>MLESKLKAPVFTARTQGRHYGEFVLEPLERGFGVTLGNPLRRILLSSIPGTAVTSVYIEDVLHEFSTIPGVKEDVVEIILNLKELVVRFLDPKMASTTLILRAEGPKEVRAGDFTPSADVEIMNPDLHIATLEEGGKLYMEVRVDRGVGYVPAERHGIKDRINAIPVDAIFSPVRRVAFQVEDTRLGQRTDLDKLTLRIWTDGSVTPLEALNQAVAILKEHLNYFANPEASLLPTPEVSKGEKRESAEEDLDLPLEELGLSTRVLHSLKEEGIESVRALLALNLKDLRNIPGIGERSLEEIRQALAKKGFTLKE[2x];> MEIKRFGRIREVIPLPPLTEIQVESYKKALQADVPPEKRENVGIQAAFKETFPIEEGDKGKGGLVLDFLEYRIGDPPFSQDECREKDLTYQAPLYARLQLIHKDTGLIKEDEVFLGHLPLMTEDGSFIINGADRVIVSQIHRSPGVYFTPDPARPGRYIASIIPLPKRGPWIDLEVEASGVVTMKVNKRKFPLVLLLRVLGYDQETLVRELSAYGDLVQGLLDEAVLAMRPEEAMVRLFTLLRPGDPPKKDKALAYLFGLLADPKRYDLGEAGRYKAEEKLGVGLSGRTLVRFEDGEFKDEVFLPTLRYLFALTAGVPGHEVDDIDHLGNRRIRTVGELMADQFRVGLARLARGVRERMVMGSPDTLTPAKLVNSRPLEAALREFFSRSQLSQFKDETNPLSSLRHKRRISALGPGGLTRERAGFDVRDVHRTHYGRICPVETPEGANIGLITSLAAYARVDALGFIRTPYRRVKNGVVTEEVVYMTASEEDRYTIAQANTPLEGDRIATDRVVARRRGEPVIVAPEEVEFMDVSPKQVFSLNTNLIPFLEHDDANRALMGSNMQTQAVPLIRAQAPVVMTGLEERVVRDSLAALYAEEDGEVVKVDGTRIAVRYEDGRLVEHPLRRYARSNQGTAFDQRPRVRVGQRVKKGDLLADGPASEEGFLALGQNVLVAIMPFDGYNFEDAIVISEELLKRDFYTSIHIERYEIEARDTKLGPERITRDIPHLSEAALRDLDEEGIVRIGAEVKPGDILVGRTSFKGEQEPSPEERLLRSIFGEKARDVKDTSLRVPPGEGGIVVGRLRLRRGDPGVELKPGVREVVRVFVAQKRKLQVGDKLANRHGNKGVVAKILPVEDMPHLPDGTPVDVILNPLGVPSRMNLGQILETHLGLAGYFLGQRYISPVFDGATEPEIKELLAEAFNLYFGKRQGEGFGVDKREKEVLARAEKLGLVSPGKSPEEQLKELFDLGKVVLYDGRTGEPFEGPIVVGQMFIMKLYHMVEDKMHARSTGPYSLITQQPLGGKAQFGGQRFGEMEVWALEAYGAAHTLQEMLTIKSDDIEGRNAAYQAIIKGEDVPEPSVPESFRVLVKELQALALDVQTLDEKDNPVDIFEGLASKR;> MKKEVRKVRIALASPEKIRSWSYGEVEKPETINYRTLKPERDGLFDERIFGPIKDYECACGKYKRQRFEGKVCERCGVEVTRSIVRRYRMGHIELATPAAHIWFVKDVPSKIGTLLDLSATELEQVLYFNKYIVLDPKGAVLDGVPVEKRQLLTDEEYRELRYGKQETYPLPAGVDALVKDGEEVVKGQELAPGVVSRMDGVALYRFPRRVRVDYLRKERAALRIPLSAWVEKEAYRPGEVLAELSEPYLFRAEESGVVELKDLAEGHLIYLRQEEEVVARYFLPAGMTPLVVEGEIVEVGQPLAEGKGLLRLPRHMTAKEVEAEEEGDSVHLTLFLEWTEPKDYKVAPHMNVIVPEGAKVQAGEKIVAAIDPEEEVIAEAEGVVHLHEPASILVVKARVYPFEDDVEVTTGDRVAPGDVLADGGKVKSEIYGRVEVDLVRNVVRVVESYDIDARMGAEAIQELLKELDLEKLERELLEEMKHPSRARRAKARKRLEVVRAFLDSGNRPEWMILEAVPVLPPDLRPMVQVD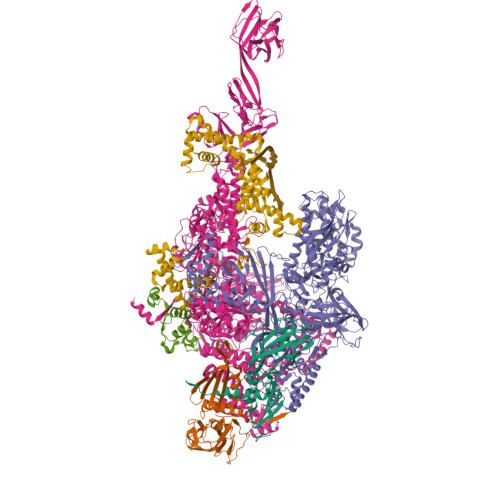GGRFATSDLNDLYRRLINRNNRLKKLLAQGAPEIIIRNEKRMLQEAVDAVIDNGRRGSPVTNPGSERPLRSLTDILSGKQGRFRQNLLGKRVDYSGRSVIVVGPQLKLHQCGLPKRMALELFKPFLLKKMEEKAIAPNVKAARRMLERQRDIKDEVWDALEEVIHGKVVLLNRAPTLHRLGIQAFQPVLVEGQSIQLHPLVCEAFNADFDGDQMAVHVPLSSFAQAEARIQMLSAHNLLSPASGEPLAKPSRDIILGLYYITQVRKEKKGAGMAFATPEEALAAYERGEVALNAPIVVAGRETSVGRLKFVFANPDEALLAVAHGLLDLQDVVTVRYLGRRLETSPGRILFARIVGEAVGDEKVAQELIQMDVPQEKNSLKDLVYQAFLRLGMEKTARLLDALKYYGFTLSTTSGITIGIDDAVIPEEKQRYLEEADRKLRQIEQAYEMGFLTDRERYDQVIQLWTETTEKVTQAVFKNFEENYPFNPLYVMAQSGARGNPQQIRQLCGMRGLMQKPSGETFEVPVRSSFREGLTVLEYFISSHGARKGGADTALRTADSGYLTRKLVDVAHEIVVREADCGTTNYISVPLFQMDEVTRTLRLRKRSDIESGLYGRVLAREVEALGRRLEEGRYLSLEDVHFLIKAAEAGEVREVPVRSPLTCQTRYGVCQKCYGYDLSMARPVSIGEAVGVVAAESIGEPGTQLTMRTFHTGGVAVGTDITQGLPRVIELFEARRPKAKAVISEIDGVVRIEEGEDRLSVFVESEGFSKEYKLPKDARLLVKDGDYVEAGQPLTRGAIDPHQLLEAKGPEAVERYLVDEIQKVYRAQGVKLHDKHIEIVVRQMLKYVEVTDPGDSRLLEGQVLEKWDVEALNERLIAEGKVPVAWKPLLMGVTKSALSTKSWLSAASFQNTTHVLTEAAIAGKKDELIGLKENVILGRLIPAGTGSDFVRFTQVVDQRTLKAIEEARKEAVEAKEKEAPRRPVRREQPGKGL;> MAEPGIDKLFGMVDSKYRLTVVVAKRAQQLLRHRFKNTVLEPEERPKMRTLEGLYDDPNAVTWAMKELLTGRLFFGENLVPEDRLQKEMERLYPTEEEA;> TSDPVRQYLHEIGQVPLLTLEEEIDLARKVEEGMEAIKKLSEATGLDQELIREVVRAKILGTARIQKIPGLKEKPDPKTVEEVDGKLKSLPKELKRYLHIAREGEAARQHLIEANLRLVVSIAKKYTGRGLSFLDLIQEGNQGLIRAVEKFEYKRRFKFSTYATWWIRQAINRAIADQARTIRIPVHMVETINKLSRTARQLQQELGREPSYEEIAEAMGPGWDAKRVEETLKIAQEPVSLETPIGDEKDSFYGDFIPDENLPSPVEAAAQSLLSEELEKALSKLSEREAMVLKLRKGLIDGREHTLEEVGAYFGVTRERIRQIENKALRKLKYHESRTRKLRDFLE> AEGKLNDELAKNKGK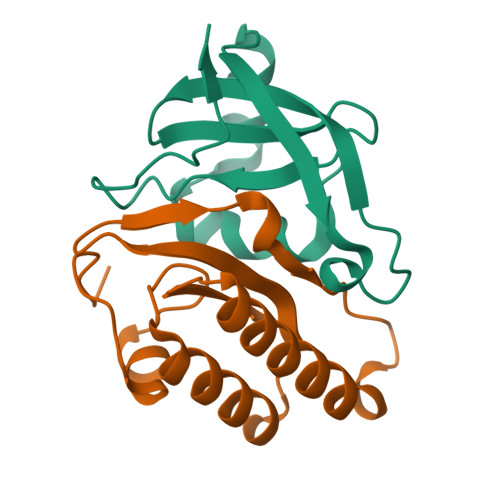IPGLKIDQKIRGQMPERGWTEDDIKNTVSNGATGTSFDKRSPKKTPPDYLGRNDPATVYGSPGKYVVVNDRTGEVTQISDKTDPGWVDDSRIQWGNKNDQ;> KLFEHTVLYDSGDAFFELKGNASMKLSPKAAIEVCNEAAKKGLWILGIDGGHWLNPGFRIDSSASWTYDMPEEYKSKIPENNRLAIENIKDDIENGYTAFIITLKM>[4x]GSMTEITFKGGPIHLKGQQINEGDFAPDFTVLDNDLNQVTLADYAGKKKLISVVPSIDTGVCDQQTRKFNSDASKEEGIVLTISADLPFAQK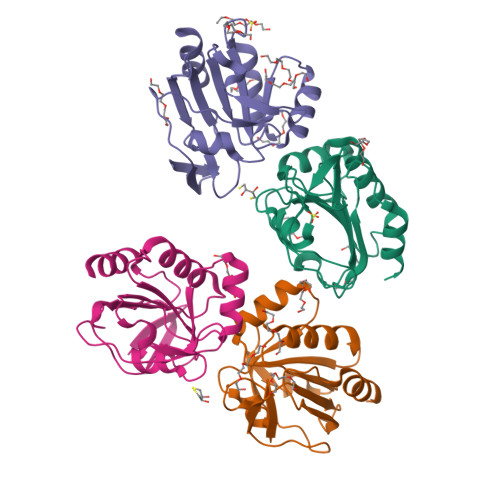RWCASAGLDNVITLSDHRDLSFGENYGVVMEELRLLARAVFVLDADNKVVYKEIVSEGTDFPDFDAALAAYKNI>[2x]GPGMKQKIVIKVPMASDKCRSKAMALVASTGGVDSVALVGDL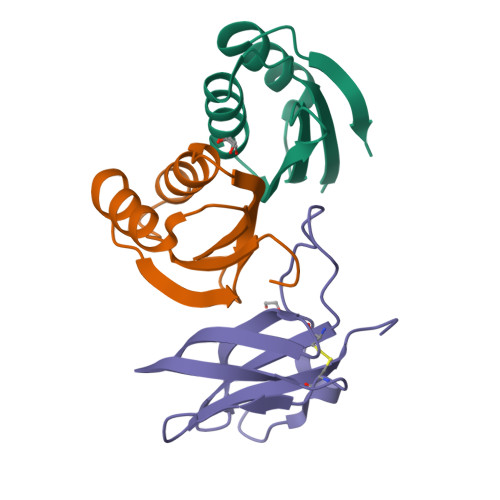RDKIEVVGDGIDSIKLVSALRKKVGHAELLQVS;> GPETGNKYIEKRAIDLSRERDPNFFDHPGIPVPECFWFMFKNNVRQDAGTCYSSWKMDMKVGPNWVHIKSDDNCNLSGDFPPGWIVLGKKRPGF>[4x]MNPETMNENGKSLKILFTALFGPGHLNACLGIGSLLRKRGHQIYFAHFPRHRATIEKHGFLFISLLDYAEPEFPIVDMLPDIGIIAKFAFERMHK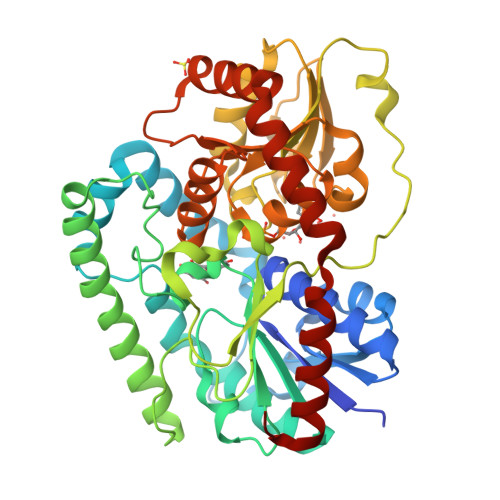LTPLELFRHASGKHTFAGMVNGSKGENYAMMKIVKEYKPDVCLADYLFNMPWMFTVDCPVIPVKSVNPIELYNGPPALTGCSIHDPPSVREEIEQLARKSELELESELEKLFAHFNVPLVSYNYAQQLGIYIYPGPLDYKELGSPKENWVRLDSSIRSTEISNFELPEKLKDKPGKLIYVSMGSLASAVTELLTMILTPLANSPHRFIVSTGPNGDSIKLYDNMWGDKFINQVALLPKVDLFITHGGSNSLIEGLTAGKPLIAIPQFGDQLDNAQRIADLGLGVRLNLHEFSGEKLLKAIEDVLNDEKINANVARVSEELKKSDSKDKVISLIEKLARDKKL> MAHMSVIQDDYVKQAEQVIRGLPKKNGDFELTTTQLRVLLSLTAQLFDEAQLSSDQNLSPALRDKVQYLRVRFVYQAGR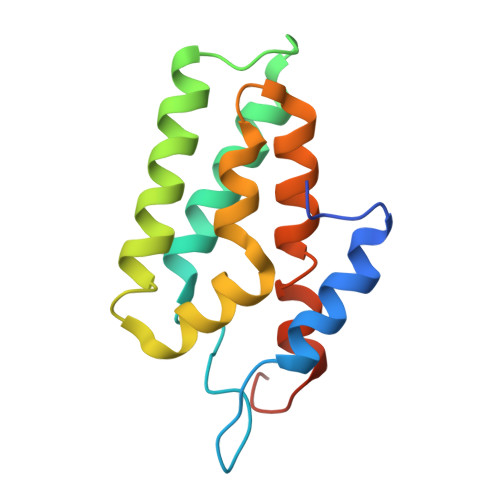EKAVRVFVERAGLLDELAQIGDSRDRLLKFCHYMEALVAYKKFLDPKETSKETE> SDEAVGDLKQALPCVAESPTVHVEVHQRGSSTAKKEDINLSVRKLLNRHNIVFGDYTWTEFDEPFLTRNVQSVSIIDTELKVKDSQPIDLSACTVALHIFQLNEDGPSSENLEEETENIIAANHWVLPAAEFHGLWDSLVYDVEVKSHLLDYVMTTLLFSDKNVNSNLITWNRVVLLHGPPGTGKTSLCKALAQKL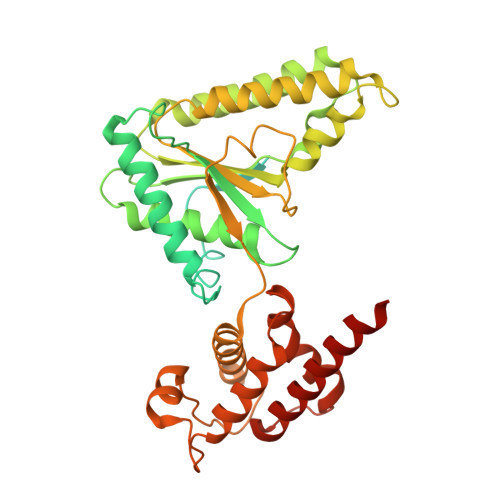TIRLSSRYRYGQLIEINSHSLFSKWFSESGKLVTKMFQKIQDLIDDKDALVFVLIDQVESLTAARNACRAGTEPSDAIRVVNAVLTQIDQIKRHSNVVILTTSNITEKIDVAFVDRADIKQYIGPPSAAAIFKIYLSCLEELMKCQIIYPRQQLLTLRELEMIGFIENNVSKLSLLLNDISRKSEGLSGRVLRKLPFLAHALYVQAPTVTIEGFLQALSLAVDKQFEERKKLAAYI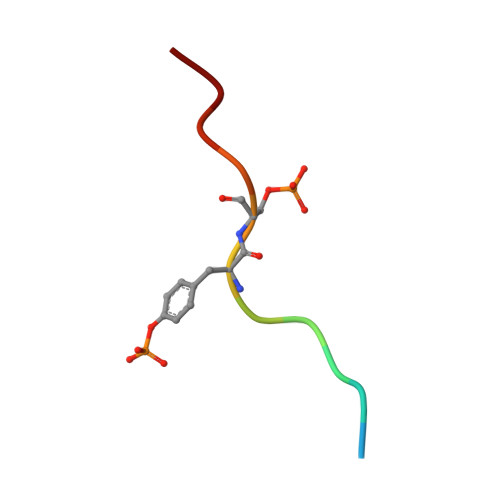> DSFLQRYSSDPT> GSHMTQEEVRKIMEKLKKAFK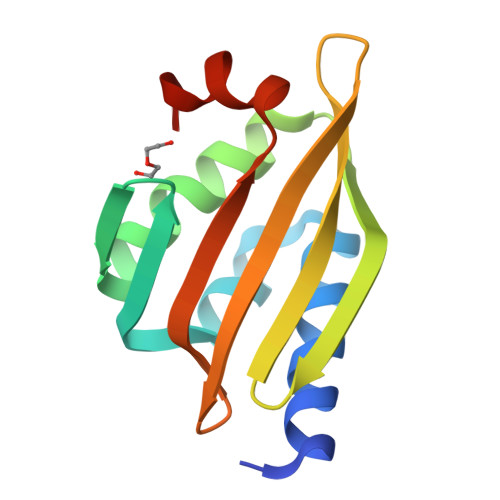QGNPEQIVSLLSPDVRVKVGNQEFSGSEEAEKMWRKLMKFVDRVEVRRVKVDENRVEIEVEFEVNGQRYSMEFHFEVENGKVRRVEIRISPTMKKLMKQILNYG4-[5-(4-METHYLPHENYL)-3-(TRIFLUOROMETHYL)-1H-PYRAZOL-1-YL]BENZENESULFONAMIDE 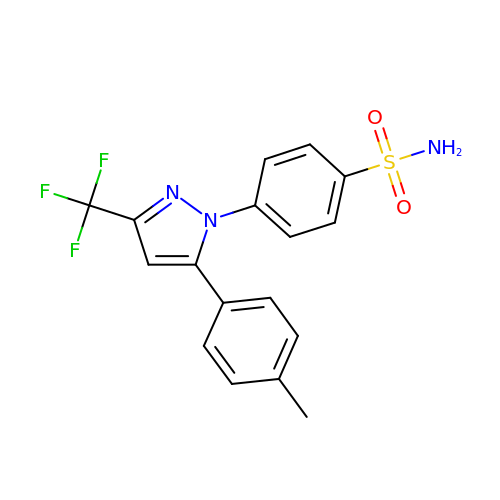| C17 H14 F3 N3 O2 S | RZEKVGVHFLEQIL-UHFFFAOYSA-N>MAHHHHHHMVTVPKLQAMREAGEKIA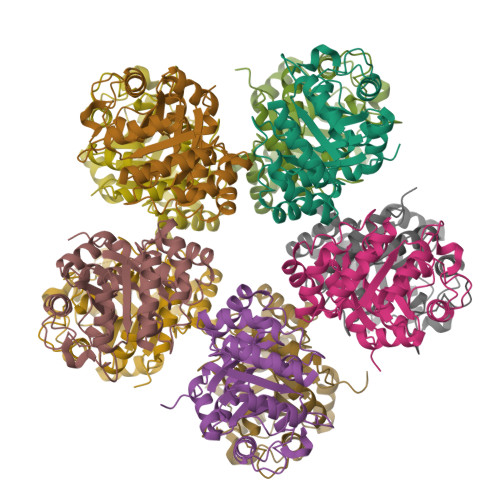MLTSYDASFAALLDRANVDVQLIGDSLGNVLQGQATTLPVTLDDIAYHTACVARAQPRGLVVADLPFGTYGTPADAFASAVKLMRAGAQMVKLEGGEWLAETVRFLVERAVPVCAHVGLTPQSVHAFGGFKVQGKTEAGAAQLLRDARAVEEAGAQLIVLEAVPTLVAAEVTRELSIPTIGIGAGAECSGQVLVLHDMLGVFPGKRPRFVKDFMQGQPSIFAAVEAYVRAVKDGSFPGPEHSF[10x]>[6x]GSVNYAAGLSPYADKGKCGLPEIFDPPEELERKVWELARLVWQ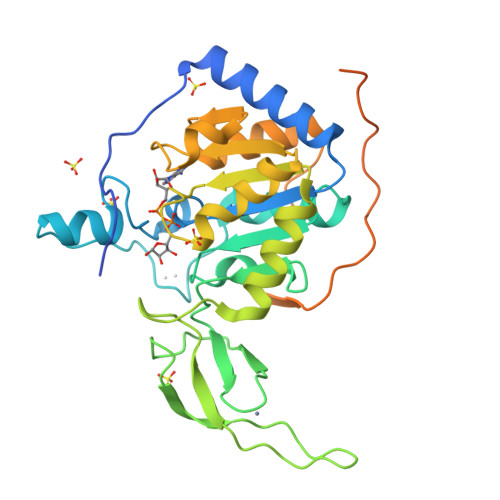SSSVVFHTGAGISTASGIPDFRGPHGVWTMEERGLAPKFDTTFESARPTQTHMALVQLERVGLLRFLVSQNVDGLHVRSGFPRDKLAELHGNMFVEECAKCKTQYVRDTVVGTMGLKATGRLCTVAKARGLRACRGELRDTILDWEDSLPDRDLALADEASRNADLSITLGTSLQIRPSGNLPLATKRRGGRLVIVNLQPTKHDRHADLRIHGYVDEVMTRLMEHLGLEIPAWDGPRVLERALPPLPRPPTPKLEPKEESPTRINGSIPAGPKQEPCAQHNGSEPASPKRERPTSPAPHRPPKRVKAKAVPS Inositol polyphosphate 1-phosphatase (INPP1) is a prototype member of metal-dependent/lithium-inhibited phosphomonoesterase protein family defined by a conserved three-dimensional core structure. Enzymes within this family function in distinct pathways including inositide signaling, gluconeogenesis, and sulfur assimilation. INPP1 catalyzes the metal-dependent hydrolysis of the phosphomonoester bond from the 1 position phosphate of Ins(1,4)P2 or Ins(1,3,4)P3 to yield inositol 4-phosphate and inositol 3,4-bisphosphate, respectively. Conserved secondary structural elements comprise juxtaposed metal binding pockets and define a shared sequence pattern of D54…E79E80…D153PID156S157T158…D317 as shown for INPP1.

Based on our crystallographic studies, we found that the lithium-sensitive, inhibitory metal binding site was coordinated by the carboxylates of two conserved residues, D54 and E80. Residue D54 was mutated to alanine, and we kinetically examined the effect of Li+ inhibition upon the wild-type and mutant enzymes. Mutant INPP1D54A exhibited a 4300-fold inactivation relative to the wild-type enzyme with a Vmax of 13.9 nmol/min/mg compared with 59.7 μmol/min/mg for the wild-type enzyme. While a large change was observed for Vmax values, the substrate affinity appeared to be relatively unaltered with Km values of 11 μM to 31 μM for the D54A mutant and wild-type enzymes. Although the D54A mutation does not significantly alter Km, there was a large effect on Ki. As mutation of D54 results in loss of INPP1 activity without significantly changing the substrate affinity, we hypothesize that the D54A mutant can be utilized to trap the substrate in INPP1. To rule out the possibility of unanticipated conformational changes, we first determined the structure of INPP1D54A in the presence of calcium. One calcium ion at metal site 1 is found in the INPP1D54A/Ca2+ structure, alongside two sulfate ions similar to those found in Gd3+ structures.

> MSDILQELLRVSEKAANIARACRQQETLFQLLIEEKKEGEKNKKFAVDFKTLAAVLVQEVIKENMENKFPGLGKKIFGEESNELTNDLGEKIIMRLGPTEEETVALLSKVLNGNKLASEALAKVVHQDVFFSDPALDSVEINIPQDILGIWVDPIDSTYQYIKGSADITPNQGIFPSGLQCVTVLIGVYDIQTGVPLMGVINQPFVSQDLHTRRWKGQCYWGLSYLGTNIHSLLPPVSTRSNSEAQSQGTQNPSSEGSCRFSVVISTSEKETIKGALSHVCGERIFRAAGAGYKSLCVILGLADIYIFSEDTTFKWDSCAAHAILRAMGGGMVDLKECLERNPDTGLDLPQLVYHVGNEGAAGVDQWANKGGLIAYRSEKQLETFLSRLLQHLAPVATHT> MGSSHHPHHHHHSSGLEVLFQGPLGSHMNTRRQQAQNIRNNAAELAANRPHPQHINNKEEYEYRRPKKDGNEPSHIANFTKGLPHDEHTGLLLNSADYDQFVLGIQSGDTTDFARTPLGPAELPKVHGCLSKQKIDCDDDHRSGFWKSQIAQGAAGGDGAKLRAWESAGAGLVFDLEGPDAQAVTMPPAPRLESPELTSEIAEVYSQALLRDIHFSQLRDPGLGDQVNACDSCPTQLSIYEAIDILNTVQIEGQNWFSANCCDLTDDEQARQRPLVTRQNIFRGIAPGDDVGPYLSQFLLIGNNALGGGVFGQEAGHIGYGAIRIDQRVRKATPCKDFMTNFETWLDVQNGADLRGLETYVDADPGKCREFPAYRVITTPRDLATYVHYDALYEAYLNACLILLGMGAPFDPGIPFQKPDVEDKQQGFAHFGGPQILTLVCEAATRGLKAVRFQKFNVHRRLRPEALGGL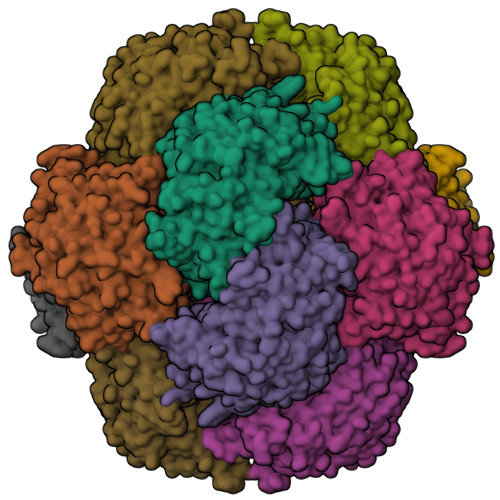VDRYKHGKGAGDELKPVAALVEALENVGLLSKVVAHNQLQNQNLDRSGDPSSAGDNYFLPMAFPEGSPMHPSYGAGHATVAGACVTMLKAFFDHGWQLNLGMANGKYISYEPNQDGSSLQQVLLDCPLTVEGELNKIAANISIGRDWAGVHYFTDYIESLRLGEKIAIGILEEQKLTYGENFTMTVPLYDGGSIQI>[2x]TNIRVAIVGYGNLGRSVEKLIAKQPDMDLVGIFSRRATLDTKTPVFDVADVDKHADDVDVLFLCMGSATDIPEQAPKFAQFACTVDTYDNHRDIPRHRQVMNEAATAAGNVALVSTGWDPGMFS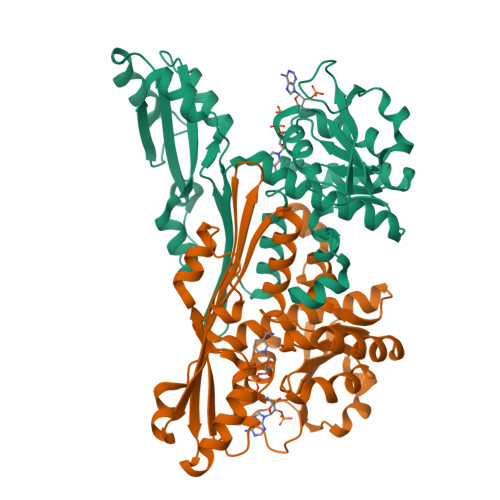INRVYAAAVLAEHQQHTFWGPGLSLGHSGALRRIPGVQKAVQYILPSEDALEKARRGEAGDLTGKQTHKMQCFVVADAADHERIENDIRTMPDYFVGYEVEVNFIDEATFDSEHTGMPNGGHVITTGDTGGFNHTVEYILKLDRNPDFTASSQIAFGRAAHRMKQQGQSGAFTVLEVAPYLLSPENLDDLIARDV>MAHHHHHHMATNITFHPGAVTQDERDTLLGQKGCTVWLTGLSASGKSTIATALEQHLLHKKLHAYRLDGDNIRFGLNKDLGFDQASRVENIRRIGEVSLLFALSSTISVTAFISPYISDRQLARELHEKHSSAIPFIEVFIDAPLSVVEQRDPKGLYKKARAGEIKDFTGISAPY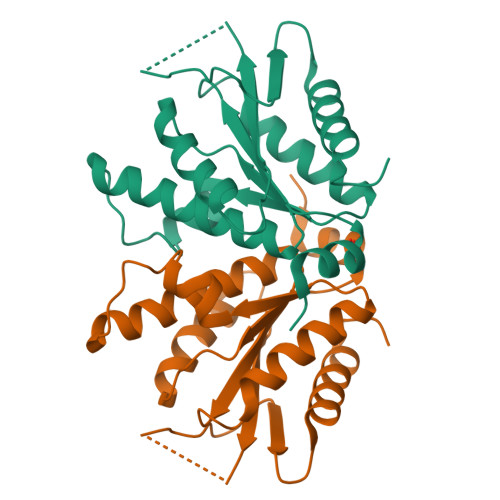EAPANPEIHIRTDEVDVAGAVEIITKYLADNGLIPA[3x]>ALALYTPLPTPTGWTTMGDVAVGDELLGADGKPTRVVAATDVMLGRPCYEVEFSDGTVIVADAAHQWPTSGGIRTS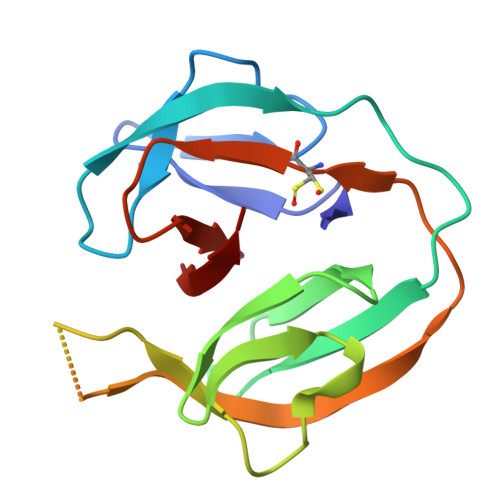AQLRSGADRIVVAGSAGGYAEQRSATGLLVPVVQIESARRVASVPVRCVEVDNPAHLYLAGRGMVPTHN[2x]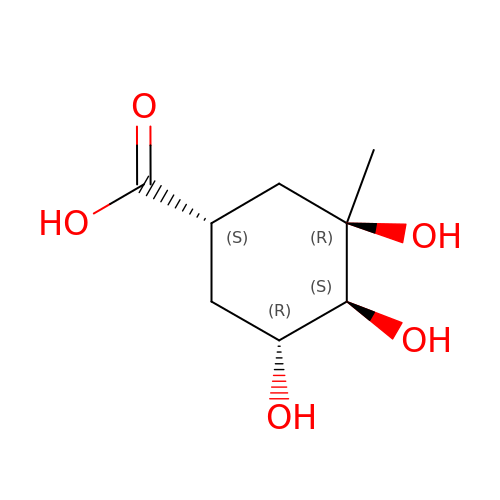(1~{S},3~{R},4~{S},5~{R})-3-methyl-3,4,5-tris(hydroxyl)cyclohexane-1-carboxylic Acid | C8 H14 O5 | OFMSIUGUPGSXKY-SKHQTKALSA-N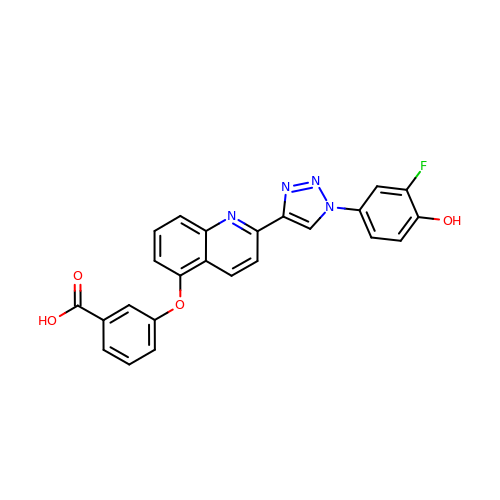3-({2-[1-(3-fluoro-4-hydroxyphenyl)-1H-1,2,3-triazol-4-yl]quinolin-5-yl}oxy)benzoic acid | C24 H15 F N4 O4 | RXHQCISHMPQZDT-UHFFFAOYSA-N APOBEC3s (A3s) are an APOBEC subfamily in mammals that restrict viruses, including retroviruses, endogenous retroelements, Hepatitis B virus, and Epstein-Barr virus. The double-domain A3G, A3F, A3D, and single-domain A3H (haplotypes II, V, and VII) are active in restricting HIV-1 through deaminase-dependent and independent modes, with A3G being most potent among them. For the double-domain A3s, the deaminase activity resides only on CD2, but the catalytically inactive CD1 is important for regulating nucleic acid binding, processivity, oligomerization, packaging into HIV virion, and effective anti-HIV activity. In order to understand the structural basis of domain organization and molecular regulation of the complex biological functions of A3G, we determined the double-domain structure of rA3G.

Two fl rA3G mutational constructs (termed FKL and E/Q) yielded well-behaved proteins and crystals in different conditions that diffracted to 2.47 and 2.40 Å, respectively. The E/Q construct was crystallized in different pH and salt conditions but consistently showed the same structure and dimerization via CD1-CD1 interactions, primarily through direct packing of several residues on h6 (K180, L184, A187), loop 1 (I26) and loop 7 (F126, W127) from both subunits. While the FKL structure shows a canonical fold of its CD2 domain, the E/Q structure shows significant alteration in CD2 conformation, with major changes on helix 2 (h2), loop 3, loop 4, and the Zn-active center. The long h2 of the CD2 in the FKL structure has become a short 310 helix (h2′) in the E/Q structure, resulting in a disordered 14-residue stretch spanning parts of loop 3 and h2 (residues A246 to E259). The shift to a short 310 h2 and extended random coil structure is necessary to avoid clashing in this tight packing conformation. However, this also disrupts the conformation of the CD2 Zn-active center within the regions of h2 and loop 3 that become disordered, resulting in no Zn-coordination. When aligning the FKL and E/Q structures via their CD1 domain, the CD2 domain of the E/Q structure shows a rotation of ~29° compared with the CD2 of FKL structure, causing the E/Q CD2 domain to shift ~15 Å downward and ~8 Å toward CD1, and resulting in a much closer packing interaction with CD1. In the E/Q structure, the two domains interact mainly through h3, h4, and h6 of CD1 with h2′, β2, loop 4 and loop 10 of CD2. Additionally, E/Q* carrying individual mutations F126Y, K180S/L184S, or CD2Δloop3 (as in FKL structure) are all active, even though the activity of the FKL* construct (with E259A reverted back to E259) with the combined mutations is less than E/Q* and WT. These results suggest that even though the crystallized E/Q structure, lacking Zn in the CD2 domain, represents a catalytically inactive A3G structural state, reverting the catalytic residue back to E259 can fully restore its deaminase activity comparable to WT.

>GPGGSGGMKPQIRNMVEPMDPRTFVSNFNNRPILSGLDTVWLCCEVKTKDPSGPPLDAKIFQGKVYPKAKYHPEMRFLRWFHKWRQLHHDQEYKVTWYVSWSPCTRCANSVATFLAKDPKVTLTIFVARLYYFWDPDYQQALRILAEAGATMKIMNYNEFQDCWNKFVDGRGKPFKPWNNLPKHYTLLQATLGELLRHLMDPGTFTSNFNNKPWVSGQHETYLCYKVERLHNDTWVPLNQHRGFLRNQAPNIHGFPKGRHAQLCFLDLIPFWKLDGQQYRVTCFTSWSPCFSCAQEMAKFISNNEHVSLCIFAARIYDDQGRYQEGLRTLHRDGAKIAMMNYSEFEYCWDTFVDRQGRPFQPWDGLDEHSQALSGRLRAILQNQGN[2x]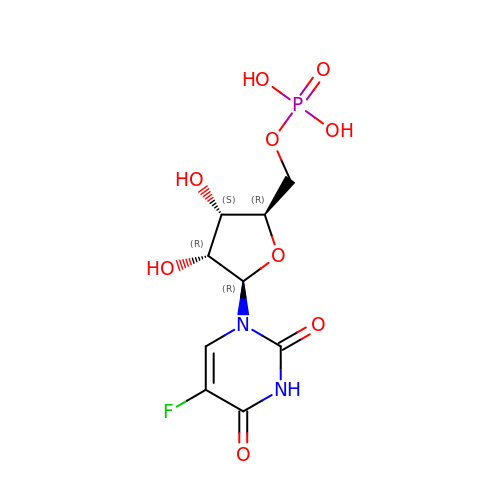5-FLUORO-URIDINE-5'-MONOPHOSPHATE | C9 H12 F N2 O9 P | RNBMPPYRHNWTMA-UAKXSSHOSA-N>PGVERTDITYNLTSDIDAAAYLEELKQNPIINNKIMNPVGQCESLMTPVSNFMNEKGFDNIRYRGIFIWDKPTEEIPTNHFAVVGNKEGKDYVFDV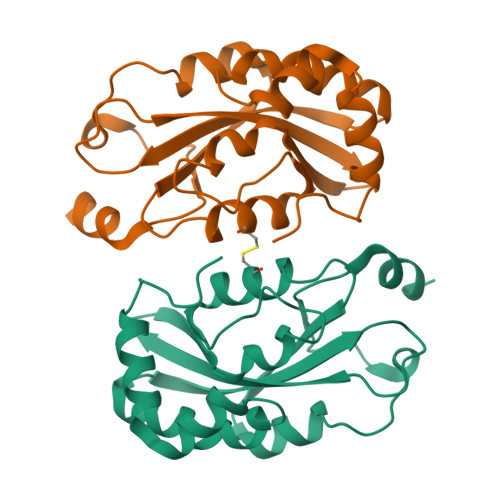SAHQFENRGMSNLNGPLILSADEWVCKYRMATRRKLIYYTDFSNSSIAANAYDALPRELESESMAGKVFVTSPRWFNTFKKQKYSLIGKM[2x]>SMGKEKSKEPRDPDQLYSTLKSILQQVKSHQSAWPFMEPVKRTEAPGYYEVIRFPMDLKTMSERLKNRYYVSKKLFMADLQRVFTNCKEYNPPES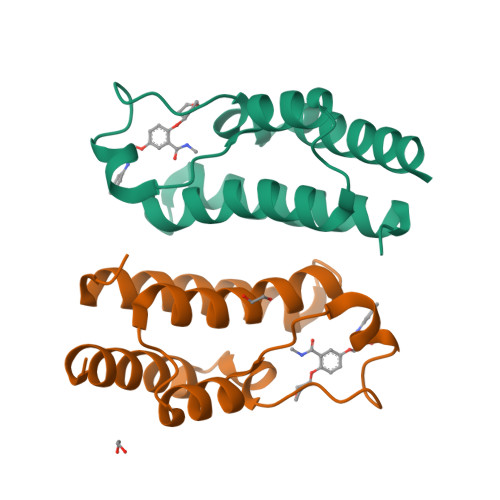EYYKCANILEKFFFSKIKEAGLID[2x]> ALTPEEYAELTASAETRSKLSEQIALCRQMLQLIELAIARREAAIAAGIPGITKDICGYDTRLDTVGAAHQFSLFLQSPQGQSIFSTRSLDNPPYVTTTIKNPEDDTPAA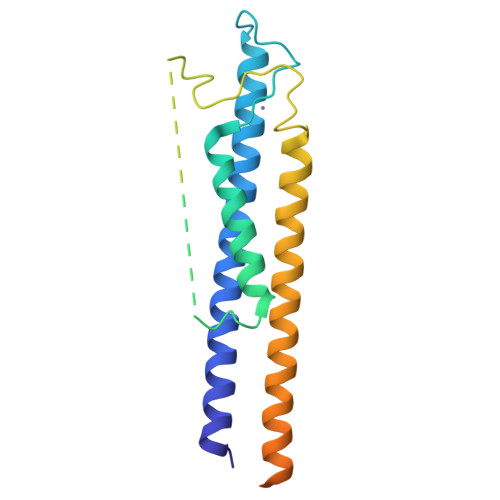TSSNSAETAAGQDPRTAGMCLRKKCKPHNGWGALLTKTVRHDIRELALQIRELLEAEQRVRDGAAGRFMRRMKERNEVIAIEEDEDDDEHGNGFLREEKLGHKRSDGDRMDLD> MTQFKEIEKTTDFKNHSLP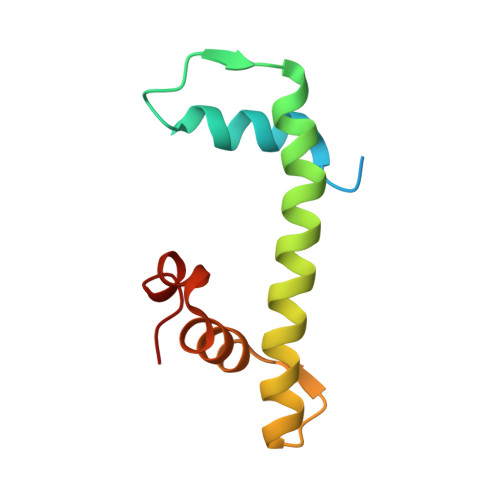LARIKKIMKADEDVRMISAEAPVVFARACEMFILELTLRSWNHTEENKRRTLQKNDIAAAVTRTDIFDFLVDIVPR> MRDMGEPKLKIVAMPSDTNPAGNIFGGWILSQIDLAGAIAARE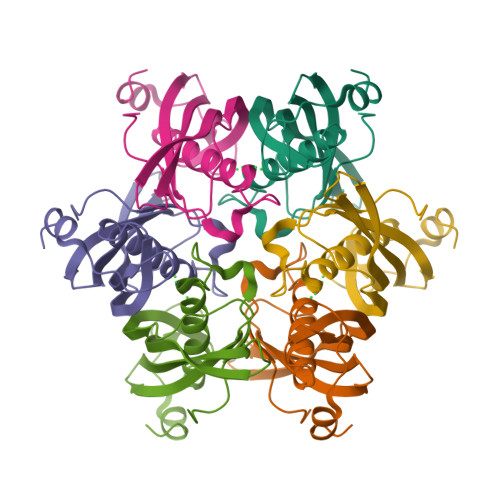LSPERVVTISMDKVVFKEPVFIGDIISCYSKVVNVGNTSISVEVEVTAQRVDSQGCTSCINVTSALVTYVSVTRDGKKNPISEELKRIHGFLNA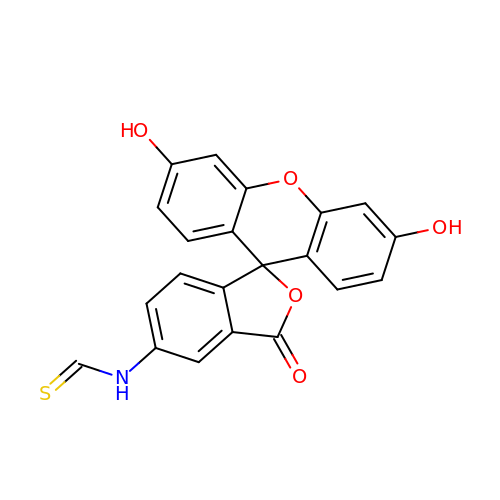N-[3',6'-bis(oxidanyl)-3-oxidanylidene-spiro[2-benzofuran-1,9'-xanthene]-5-yl]methanethioamide | C21 H13 N O5 S | XXJHFVNZDWPRIR-UHFFFAOYSA-N prop-2-en-1-yl 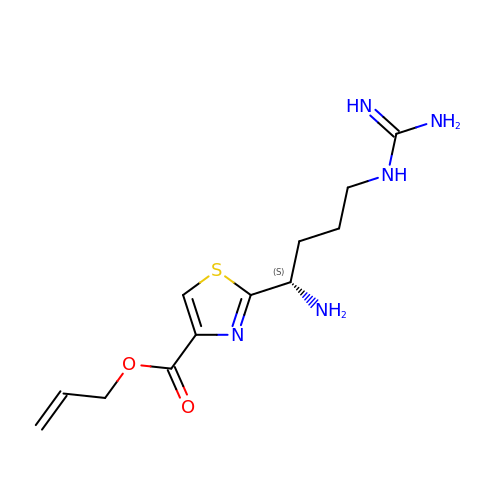2-[(1S)-1-amino-4-carbamimidamidobutyl]-1,3-thiazole-4-carboxylate | C12 H19 N5 O2 S | QJCBJWZIVFJHDU-QMMMGPOBSA-N(2S)-6-[(4-fluorobenzyl)amino]-2-[(2R)-2-(4-fluorophenyl)-2-methoxyethyl]-N-hydroxyhexanamide | 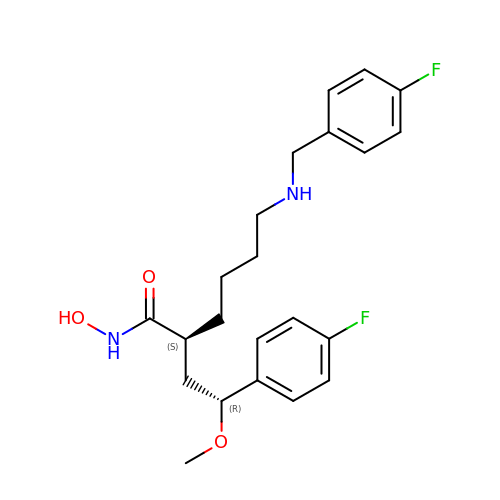C22 H28 F2 N2 O3 | SZPWYHRMRFNOHH-GHTZIAJQSA-N>[2x]MMAKAKALIPDNGRAGADEGNRQAWIGQEVLRREDRRLLTGTATFAGDLGVPGQLHMRIVRSTQAHARIVSIDATEAEKTPGVRMVITSEHTRHLGSVLLEELGYHEIYENIEDFSHPVLAVDKVLYVGQPVVAVLAVDPYLAEDAAELVSIEYEPLPVLLDPEEALTGKVELFPGRGNEGARIKKAYGDIDRAFAEAEHVIRHKYVTNRHSGVPMEPRAVVVQPDPARDTLFIWGTVHVHDNRRIIAKMLNLPEVNVRMKHVEIGGSFGVKGGVFPENVVAAWAARTLGVPIKWTEDRVEHMTSTSHAREMVHKLELALDAEGRILGMKDEIFHNHGAY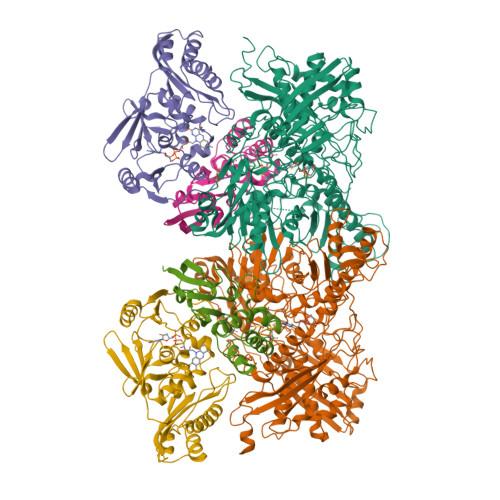FRQAEPLVSDITAGIVFGPYRVPAYDATLHAVFTNKTPVGAYRAPGRYESTFARERIFDLACAEIGLSKTEFRRRNLLTAEDLPWTPGLDIVHEPYHFDSGDVVKHFNEALEAANFSEWLEESKRLRADGRKVGVGLGVLMDKAGLGLFETGGVEVSRAGRVTVKTGGSSVGQGIETVLAQIVAEELQIAPENIDIVHSDTELIPDGVGSWSSRSTVLAGGAARKAALAVVEKARRLASEMLEADPDDLELTAGSFKVKGTDQQISLYEIAAARDPFTARADNDEPGLAADAVYMNNAMNYPYGVTLVQIELDPDTGGHRILRFSTSTEAGRVINPLTTRGQIIGAAVQGIGGALYEEFLYEEDGQPITTSFMDYLLPSAQEMPNVDCFVTEDAKSPDNPFGAKGLGEIGIIAAGAAIASAIDDAIADGVHTDRLPVTPEQIFSRCQGLNKAER;> MKPPSFDYVVADSVEHALRLLADGGDDAKIIAGGQSLVPLLNFRMSRPSLLVDINRVPGLANIRKSDQTIAIGALTRHAKLTTSKTISQNLPILSEAAAWIAHPQIRNRGTIGGSLAHADAAAELPVVLLALDAYVTAQSLQGERKIPLKELLVSHFVSSILPGELIVEVNVPQLPHGSGAAFDEFSRRHGDYAIGGAASIVTLDEQGKCSRARITVLGGGSTAIRCQEAENILIDSTLSSHDIAAAAHAAVQGLDPVPTVHGSAQYRAQVIRTMVERTLAKALHRARPTKESMDH;>MNAFRLTVEVNGVTHATDVEPRRLLADFLRDDLHLRGTRVGCEHGVCGSCTVILDGQPVRSCTVLAVQANNSRIETVESLQKDGQLHPLQRSFSKCHALQCGFCTSGFLMTLKPLYDDEDVTLDATSAREAISGNLCRCTGYQQIVEATVDAFHCRDHND[2x];> MKPPSFDYVVADSVEHALRLLADGGDDAKIIAGGQSLVPLLNFRMSRPSLLVDINRVPGLANIRKSDQTIAIGALTRHAKLTTSKTISQNLPILSEAAAWIAHPQIRNRGTIGGSLAHADAAAELPVVLLALDAYVTAQSLQGERKIPLKELLVSHFVSSILPGELIVEVNVPQLPHGSGAAFDEFSRRHGDYAIGGAASLVTLDEQGKCSRARITVLGGGSTAIRCQEAENILIDSTLSSHDIAAAAHAAVQGLDPVPTVHGSAQYRAQVIRTMVERTLAKALHRARPTKESMDH> MFLIHFVHYKTILQKYTFKFKHIFLSIDKYNSLFFNISGILIWLNIIHINIILIKYSFFILINNFEYLIILIST;> MFRLTAASQKNLNSWYTKGTMRGGVPRIYYAWMRPGSFTRRRFEKMRNPFVDLETGTSLYFRDTRDSAEAIAHAADSKGIKGMDNAIDLYNEYRIVPDLYPEGFQWKHKLNTEYNQWRSNTWLTPDLIPKEHRGRFLCNFQLNIVAYDMRVVKFSPKDHRQWIYCVLYVGSGKGIAGWGRAVAPSTQEAKKEAIREAFSNIIAVDLEQEGPMYPVRVNADGVRVLLYPARRIVANFRVADILCAFGFQH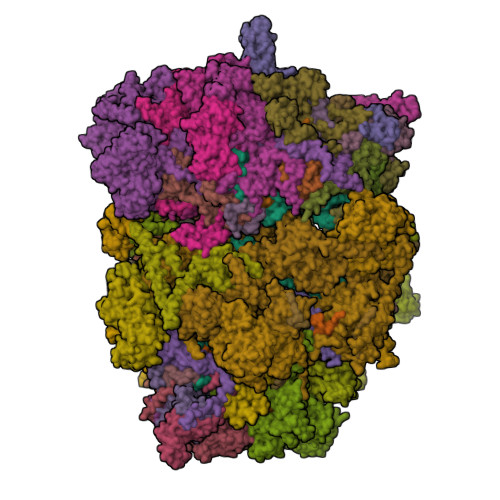AGCRINLKATNNPKSPTHTVEGVFEAVKALRSVSEIAASRGKVPHSLIYNIYPYLEEIRRRKGMMAMHPPGKDGLLMPDRVVDNRLPDHLKRGYYDDVYWKDFFAGSDEHLNEPRMGLRGDEMRRRLEEAQTSPAPTTAKDTRRRTLEDVLKRLGKTTRDLGSIPIVNPRVDVGLPTHIKRNYQLH;> MVFYSFVLVMKPRQRRFTSQALREIGVAVYSNGGLIRSITNEGIMRPYSRFRDADNTPLTYARYIILQLDMGEEEMGKVDKIIREHQDVLMALKLNNLERPVGIRSGNKELQAAYFPLDTFTRLEEEINWSPQTSADIYTQLEMNWKEFSRTRWSSFLRN;> MLRQSLLSLAKVYGAVPPLGAAQGHRLLHGKREREGSLFAVANDVKRDERLLRQQLNALLEEERMPMQARLQRNEAVSSHEAVPQTPLVDLPGVERRRDLPADPITRLFFQHKGDHALYYGTYDKPSVQDDDRVQIEKRVPRRREENLYTPIYDFCHRIREATEQRKRFVVVPSTIETRGCARVMHDHGLVAGFRDFHNDRAFAVELKYFQGDSTINVIEPCSYDGRTEFEWSPKMMRRLLNTHGIHNRLVVYICRTADNRIIDHIHAVKENIGGRGLMMVH;> MQKLLSPRTARHARLFRLAGKLADSGSPGVPKSDGERLVWVNSHVRRDKDISLSQEEERIRELMMPLEVGENSFAANGQATHGNLFYFREYPMYPGEYVPAEHNTLSSLRDELRLDLTAQSLKEAWMRVSGGVYFQSVDEYYASVDGLDAEQIGEVLAALFPELNCYEAQALVQRTLECISRPVSAASRQLSRTITAEAVGLDNAPGHYTNFLEWMGRLTETRAFKTEHALFEFSRRKFNRDDVRVMFENYRLMSKATLLADSADSYSHFYTVLKDFARKVAGEDSRHQIGVRIDEAEVDPETGIAVGRGCADGEKYHFTALLRENRDHNGIITVMGKPLSLVLDNKAWLMEMVLMPFDEANLDYRDFDAHIVSEGHAMPSIANEIAAFALRMAVANALVKLIPLTRIPLKKSGLLSVDRRRERGQFPGYLDGKKVKRRFAKR;> MVRRSHVVAYYWSRYRMPTQMPKFDGPAPVAAPQSMNSTKTNEFIDPIDDKFPMSIRGPLVRPDVPEDQYVDSWYICTSMTHHMGDYRPWSASAPPNAFRFRPFNEFDAKGREYVQYMREFARFDPRKSRGNGQKGFPFRDAYLTKMNEANQKTPPPTLETIMDRAVREHHQHARILSPLEVQRDVGRLEPIPSYAGKINADRSVFPFQWKTEDWYEYEVAKVRNRRFVFENTEEDGIRGSEVTYKIVLEGFWDHHVMKLAEDVCMFLKDVGRQIVEEKLVAVRRLLQGGAVDPELLAAFNCARAGPFGGLDEYDKEEVANFLRSDLRRLEEQCLSVINRCNVPVPGATNIYDPHTSWPHVEKLEPWVRMAEFWTSSSDTSFTELEMSTAHYEFRKFFRVIICKLPFQSTEFEKRMYDIRHWLHRQTSCEFHTIYRRNVIHDSAVFPTEHDPATPTTHEHHRMFSFALDWQSAPVNRLSTDTVHEGESWDAVAQRLGCSVGELKDANAERETIEAGVVINVPVTATRRLTSFGATPLVLPLKTTSAKDGERIRTWEEAAAILDCTVEELQQCNGHAALTYQKKESEAGEFDSSVTELVAPLSCWTSTSESEFSPVERVHANDTLVAIARRLQCSEEALRAVNDGITDVSGLDFVRVPPEARRPRRLVEPQLRPQAATDALLARTIAEEETFKLKSIPHLPQNAERFPHEYHTPTSRFPPTPSETPATQDWMAYTAKYLDKQFTISAEPAPVYNVNKLWPMQQIPGKVDQTPFEEDQTWLLHSIPVQQLEMHHHEKDLQDLPFINHEQFPRSLEWNAP;> MMRKSVTFLRRGKPRPRAGMFPDKYRRVPMLLKPQQGGQQYFNHFLIRSTNDRLTQQDVDNASGQAHSFISPQLPQMDWRNMSARSSEESIREEMRQLAENDVMQHQRVFNERMWYEKEEEHRMKARSCPEETSEHAXSNDGAVPPPRVLGGDYFKTRFGYSLVKNSEMTQGPVDYSQLDMWGEMPRYTSDMVFLYLVSRRRNTYAVAYTYEGKRILNTYTAGNRGLKGGDRGFRSEGSTDNGHQVTSMYLNDLLPKLREMRASEGRPMGRGEKVELVVRVMGFYNGRQGAVRAVQDRANEFHVRYFEDITPFPLNGPKMPRGVFK;> LFFLRMWFLYGCCLRFVLFVLCYYMSPRLPSSGNRRVLYAVFYLYNFVWMLRCFFCCFIGLVMSLFIIEGGGFVDLPGVKYYTRIVS;> MFCFSRGLWMRHIGQDVPKRHTHFVLESRLMYEKSFRDCWLHSVCRAISQLDEPLSKTVVGTHQKMLQRKVTCFQYNQYGLFKTPYYRLANVDRYHAVQGVAGTREWVPYVNVSYWTMNKMVRGGNLLVHRVHYTGWGTDSHLKKGGWEHRWNKVLQRNVLQYSRI;> MFVRSFCFLRKYGSKSKTPDLKTSFTKTTNFRKAEKISITTTDGEIVKGRGKIRRRTHSALKEAIGAMEHPAIWLWYPWRMNPEPPTPHMPQRRALKNVHGAVFNDLTPVQKKRQEQMLYGVNIPETRQMKFEEQHPLLAGALRKLEGQPKGFPFWYRKYPTRRHAYEYRFSIPVEMLDGYNDDVKKALSKGMMSIQEKQFAQEAMYMERYAEHDFDTTSPAVLAVKRALKCRVLRNHLLTNPHNNIIKTVLANTERKLNHALRRLRKVDFKKYWEIIRDHDVQDILQPPNLVTYRQGSYWKYDWNAGLAISTNLADVMDPRGLNGCVETGRSRSEVARDLGLSYTRPLHENEKKQLSHQAVYYERLAKFKMEQPEAARAMERERFVRKFSGMFVKMDIRSGAPDFPSTYRRLLGTKVVRWASKRHGPN;> MQVTETVLARAVIKRRSPQLWGAPGAPIIRMRGHHVVWKFQSYDLVVEHTHKRRNSDIRLLHYLGKHCPHPQKSLWSPDTPVAQDRHLFMLTTVDIDAFKYWFGVKRCRLSMKPWALLAKAGLLPPSLTQNSKIMPKPLFDKESLMRYYLANRKDEDVMAREKYLNYENSMVKTEEERAAERPVAPYL;> MLRRSLLAFPWWNFQTEHRQRCVLMYGGARTKNTHNANHRVFIKKYKRNAFPNRTRHHWAVSMTGVLSQRPRRMPWPYDLTSLIFNQPRQGSDKIGYVVGTSMLKTAVVATNHMVYYPKFNQRVSRTKRFFAHDEDLACVEGDLVHIKQCRKISKYKHYYVFSILEPNVEGRERLKLGLKAVPPPLFGYPVSRRIVKLNLTSTEGTQEKLAAAIQEHVQDAYRFSGPTPDQPRNRLADPVTFEDANNMIAPNAPAAAALDASDSPPLLDRGEYTEVEQDTRNKKGDDYWMNLQPKEKYDFKSFKKSP;> MNRTGGSIYAHALSQFAVCRQPWNEYIGLLTKQDSTPYHTEPQEKPAYRGRKQGREGWLFGQQVQLHYHRFPDEQLITNLSRWRTGETVGDIAMQQFRNAQPFDIEDKDPQGVQRPSPEVYMKLNYKNPATISRFLTRTGHMYPADILPLNPEAVVKLRVAKAQAIRIGLYPRFGNPFWFRSQKFRPKAYQENYDPTTYSTKRTVEHFAYNWVQTDRIRRYFRELEAVHTSGSASARGSGGGTTAEHKQQDQFYSPENQPISLHRNNISYMEDVGRSVKNPTVPGLMSTKGMKKKFHNLYSSTSTKRMGFSNPTLGIKKV;> MAFRNTFTTPGKFSTVSKNIVLLLIWRVKVFLRAEGFAHSLVMLPVSLYSKILLCDVKKKIVYFHCCTRKKSMLRRCPCVWPDGPTKSSVSIGTAFTLQKRFLKIAKSAFGFYLARRGQRKYPFLRRPHIKNTHSMNPSAPYFWSFMTAKSQMAFLPEENYITGDWTGKFFVSKRQVYTLQHATSGAKVRVKSFPSIFEFNSPSRWNIGKEMNTLTKPRMDLIDEQMLTKKQRLDYVRAGLLPK;> MLHTTRLWLGGYMMYHRKAMGTMKYSKWKGAHGGISHFYGRTPMVEEVRPNEPITLVDRRIMHYVHHSRLRHFQLFRSYQEKSNSTECKLREGEMLRRRWHRRLQKSFIAFMQFKTMKVLEDQARLVNTYGQAAVNAALGDPWNATDNVARERKSAAVRRQVRALPMVNVVPKHVATMKQIHNDRFNYRWRVN;> MLRRAYIQRRYPFNKRGPREHKSWKHHVLTEPPKPLQWRDPKVWTRDLSVMKSFDAPQWDLWQSRPRSEDMDEALQPFMDMPKSLKDRRYDIPWWANPFGAWYLQNILSLELLKLKSKTNAEKIATYRSYMRSLASGKDNTMSDDDVIRNIIKERWKTLEFGDRNAGYPCTFGDYIQFLNEWFKSLDEEGMQRLREHFDRRIRPLLAVMSPVDILWLEALTQNSPHNKEQLQRKIAFQTSLGTPEFFDMSKRLRYEINEDYKVRDELGPELFALWSKAPERWPPERLSKMYGLDFTLVRKILVWHHFKACYDACVEPDWSLPKRLFALEWIRDVRARKHGLFYGKMRFAEQKITFYSDRFLFRDLVNRREASYANVWEMDDPYRFLQTEQDYEDYWGDNYDVYRRMFPEMIGRTGEPVQQYGQMPIWAGPHRQHANKSEHNWMFAEIGVNVGHEALKKLELDPTNEKRRRFVIRQPDGTLRSAKMSEMRAWYWKEEWADFRFWAPQMEWGIENTPSQEQYQEHVPDTTDADFRKQRRIQSRPVKWFYESHYTRTGSFAGFQPLRFMQRRTEREVRWPDVINAAVQIQKRKPAAYIFKAIPEL;> MRQCVVRRYKMPKNMGVAPRFDTWNEKYEPWEHMKRMGRLVGTGFYIPPEWYNHFRMFPPINHNFQQEKTLNPHNASEPTQDDTSTLSPERVALRDELARKSRLVASEGMRYYNIFWVRKPLDTMEKEYYELKRRGVDHGEAIRKVLQGFYSGLAVKKRVAAIQAEEAKLTGRFITMREATVVLGVLAKLHKEQLTPHQVSLLAKEQGETTQSGAKLTAIVSRTQPHVNKEASSPATSEAVGSSTEESLSADALASMLSEDGEQSAVGTRYQVEVKETANDSVRQLREKAEDQTGFPDWYTGESPTYSGTSXCSRDGFALMKANK;> MMRSSSFCRRQIRPYYNLPSKSEHGRKMTGFLTPYRHWMWKQNELWRNVHEAQFEHLRRVYKRQWLESFRVNADEYIYKYNITKAAQLAQWECEMKEQEKKRIEARQMMDGRQALKKKHLDLLREFHERQFFFWYERASERLQNMNLINYVPHAQLREHIDKELDKYVAGKNEPYPLNFVGQMPFLEDGDGNIVEVPESLLSNHMAEHPDSTAKPHEPHTSSSISEAAAFEERMLRAMVSAKEEDLKEWLGDDSRALSETIDDISREEEEREADIRVARSMEETDAEREVSRRAYIERXKTGSRSIFRPPTVSEGAGGTPSAPAGDANTPMRRRKKGKLDRVHALQAHQDELLAKLSSQGLKEXVDASSVPERGKIVQSRGRIRDKAVIPTHEVLMQKPELAAGSTPGARIQTKDMVDKMYHRGKYKKSGSGDKSDGEDL;> MRSKTLKKSLAAMYMRPPVTCYTDACEAPVAMWDGAIPLKETRKLKNGVPVRTVSRTYSHPPQLTPTQLSFNDINSMYCVGNDELIQFFPEGLGGRVFQTMPPGHPRGFLYRKETHLLNLFVDKVQHWHTKRSVLSSLTNGRTGFIVDGPTGCGKSALMCQVVHFARSRNIVTLYVPDAKVWTHGEWCWPSTILPGFFDAPDAARSFLKYFAVANRATLTSWKLRCTPKDLPTEQGERQPQNLYELCEWGHRAVAPASIDRQSVCVKFLMDELSEEKKLPVVIVVDGWNLFSHETHFRYPHPDFLRGLASFNESSTDIDLYPQELPRIPASRLSFVRGLNKMILSGDDPNKFFITCTTRDFKPFDGISGFPNVETDRFANSLDEYAPYDPEKDSHFHPIQIGNFDEYEYRSFLRFLINSGELAGLGWGPLWHASSDFERKLYKIGFLSGRNPQGVVDHYHQELVWRYDYQRTRQKQYLLKRRMEGMSRGASSGAVGVR;> MVLRRWFPLLGVHRVGYTHPSTLPVPCAQRWDLRLARARIFQEYIEEKAPGAWQLEDERSMSPEFKTFTGYPMRDMRPGYGQNLPDYIMKKRLPNNTHYELFARRDIPNEDNAMYGKYLYDMTVHGTSLPSTYRMHKDINKAQRNDRKLSGNRFKVLCSSGAKNPPSGWEPIPDATEEEED;> MLRCARVALRADPLNGGSSMTLGSKGSKLSPEPHRRRMPWTAAKEYVPGVVLNARDKMVLDGVQLLDIESIDRASQLDPLEVLRAVVATREYNISTGKNIFQLASQATYNGRGQRFYRKEWQEGTYDKYVTLSAIDFDRDGNKGTAYGYITFHGETTTRPVQVDFADVPGWYMDFVEERAVPFTGIVPPPPSIGTDVPVDPHSYRLKAYPYYDAPNPPEFVERLLKDRGVLPDTPTETADVDKDPTTSDGSVHYDGK;> MRRWHRSLNPALFGERGSGHYFSTTRARLQLQAQDRIICGTHGAGIVAHQTAVNSSDNPMLSSVTTAAPAADLSRTKPHEGTGTSERDPYIRTLHNQRSAAPESSVSQSHTVNAPTVDECEMLAERWGTMNYWHNDTFPRLVVFLKKLLVPDVSPLSPTAESLLSMFEKVVIPKLTSDEEDRRKLVSLWSETTLQAEAAVTKFLFQRGSFESMLHRIITDALEKMSTLALGGQEGNLALEALKRQTLFKRNDYIQKRLIDVVSNSAYLGYGDSVWQVFFAAVEANEENLLSDRATTDAIRAAWEGVMREDVVRLPDVTGVVALYLTLVCIRESGRLVPEELKELSSGLEDGVRPGVRKLQQYPLIFLHPTVKRRFVVKAVAEILHNSSSNAFSNMLRENGLHDTAREVALCEAMNRNKELAEGDVGDAVGRFVSKGEVKTLLSSLVSGTDAVVRDAVAGIFGIGTTITIDWDAVMQNVDWSNNWQRLATALLSNSAVLSAIVKLVKNAIGAKGMSKHLFTDEYADQLQLILDAREERAASRKQRIENIAQELSSFERVDLSCDLLRKLGVDMTELDTAAAATRNMNVVQRPCIEDGLLSLVLEAVTKRHPNWVKAGVIQTTLKDPFDALRWMMHIFIRLSYVPHAGAATIARLSRRRIGPIGLEPHQFNVPAELGFVEQYDNLQYKRYDWQGWYQRMLDVHNRNVSLRCRICDLQRLDGNGVQFVDMQTERRLRILAQHRVGMGVLKLDADKYEDQADNVTFGTTKLSELLADARKAQLGEEYWPSVELKVRKPSGQSKAHYSLIDNERIEKRSGELYEKYRDAKKRSLFVTPMETWLEVKGMQVRKSVDNADEDGYTLDALQDMMDGDDGDKV;> MKSSDIFFAYRLTPVVFKSRQHDSGVNQYGLKPTNAYDYINPTNLINFGRGTTFDNLGVRRAGRGEIDSSPSHSGSPVFTQAKLIGLSGEEQLTMCQSETMALRLCMAKAGKETCERESRALDSCLGRVGHLRRAMSEACWEFNDWFIQNVSDNHTKPFQHRPHDWRHFYAQEKLVRERQQNGHAYGRRPKQFSFGARYVKTDGYGKRPRLPYNK;> MRAGCVACSRIPKLGIAALGSTTTSMQATCQETQELRCATTQMAPAVIFPLPPPLRGSYIDRKPTAASFNEHHATASFRHHMIASADVSHRPRHFYFASGTRNDTGTRSVKEGERKQLKQQTNVEVDSVAYGDQLDELSARWAAKFYGQVTFGPRNYPYPSSRWLARRFQMKKHRIIKRFRFRRYKLAAVANLPFAKMIRVGMLPELKSSKTKRGDVVDPTLSGQLVSAVKNTGEKRKGQRTRPKSKYQV;> MLKRTLTVLDQTYGPHKSYKYTYMPDPRKLAPIETTQRSEIVPQSIRPPTSYVPNHETFLERADIHRLRPTSDFKASFKDWNDLFTCDKRQLRVRGIPRMTRDAIRTAVQAFQNGNPPERFDTKEEWLYYKQFKTVDYSYRVIPELPEKYRPHQSGIDQAPLPDYREINKMPQWAECEERRQSKKTV;> MIRRRVCDGARLAPNIRATFSAVRYQSGLHTFIRDSKPSNFSSVRRSENANGDATASPGATAGENPASSGDWASHMQRELFGEVDPLGGQAHKDYYRDVTRGYSPQYAPRNFANGGAVAYPHIQSPYEYEEAAHRRVWLDHDVDRMREEFTQHRASLRSLASAQEREELLRSRAAEYQVANTVHESESVHPIQQLYNSGGTSRSALKQQAVADRYSIAEQHSPLPLTTGVDRDALDEAQRTKDRILNDSFTAENLLITHGLREKEKHDFTILQRTVRIPFQGYDMDRFLAQQKGTPYGAQQLPPNVVPSSMEEAQRTLRGSSATATPLVDAVAQKVYARNTVVDRPAIGEQLTEQIINIMRASRTTAEQQREEERAQRFGLGRQGALVQDGGPDQRTLKKHTNDERIVDAMLFQQNAYRKTPTDEHWNPYIRRSTENGVGHLLQNKFDIMRREDRLSKGEQDLTERNTIHYGVPIQQIVDEFVFRHRNARGERPLDYFKPFPNFRALRLNRMYRDVEGFSLMKQRPEFLEWELFTRYRQHHQQRRRLALLHGLEPVANETAQERDTRRHRLDEICERTPFDEREMRVNDDEMRVSVETLRSWFGVYMLPSPTVVNAVLGGSASVNLHLYHLADEMGTADTREHVLSSRYLNRLLLLESYQNRVGRGFMNHVVGRAPEPVVPHEQPQEVLRHFSAEERAMYEQHVKEQTSRQLGEWERAMKRRRWLTDHQQYGHVVSHGLETSVVDLSHTETGAVLTVSTKAYEQEIEAVRMKTNATIKVDGMVYNLLPNSERRVVPLTVQLDSGEKIDMTSEDFDRCELEAFPRNLNHALNYGIANYAYNRGNYVETQDSIWEEQTASGQEGWSPATHADGLREGLPVRARRPIFSSSAEQRIAGGPQRAVIIQYHHQPFFNPEPRLVKVAFQCDGTIMEVPISDVMIWQRRYHGPERTVGDESRRYNPAAMRRYVDVTDPFNEKTSNTEHFLDKYEPKRNADTVADKYRTTKQITEIDKWTRYDSARADNYRPLSISHRRDYIRMGYIPRYTPWEWIAIQEADQPLIAEQIRQDNIGTSYFFSLNRYWRYKASPHGYIRHFENEVRDLLQYVDGVTPWKQAQKIRTYWEVRSHHPMPQFNRPEVAMHRNTVGLLPAHMWETDKKTGKVKSVKDSVRDYQTKTPYPKWVQL;> MFRVRRLAGFIQCSPCGKMGPLKQQTRRYTPIWKSDPAVDNVAPLRDEDERRALWAEVGPISDVGSAVTAWIRFGNDPVLHTAVPTMLGGKFRNQQREKESLLPNSSSPFAYVEDYMGTNLVFGSPVHAKESAAVWATYFERRYASRLRLSRRTVANYVGLINSPEVFDDESDRPETRWSQDTFFRECAYLSEKFLKEKVSNMQQFEAALKRASPEAYLAFFDAFQQQTQTQIPLPSPSVWHYEGERRKQWAEKFISISHKAQAFFKDVLSEDVKKYQEVPGKLLQKVKPVLADVGKILVKRHERWLKGRVWTSLTEEEREAYCMKEVKRQQMQVEDGEFDPMMEDDVDDTELEEWQREHDAIMKLMNSPIDGLHFTTLELWLHTMRCEELETEHIYTSARVRAIQVAARKKLYDTTSYEEVIQAVVESIARGTLDLGAGVLRPHFNEVWCQLNYAKFGSSTITQHTTTSRRQLLFFHAGSLKDIAATATLYYATKPLSNSLDYASPYKYRRSLITLCSNYGVETAYTTQRPLLRSAANLARAEDLIHAVVTAAAQPFGERRRAATRDLHMEFQRLAVPVERVIVANPVSALLESGADPDEKPVEGEKVNMWPLGAKRVVLYKWSAPNVEKLKAMESDAASAVSGSSLTAKRLREIQELKRRGFLEVSLWRRVTAQERKQRNEIVEAKKKQVEEVVRTVPSLAHLHQYATSLYSRIEERVAFPTETSTVTETTNMKEETNKPLEDSEWEFAVLLDDRVLLNKEESVELYLPYRDANGELLAQGEYRALVRAFDLEANPNLHPAYCSVGYSESFQVFDALPQLIAQFFRVKDATAEAAGVTHIPAADFTPFCAFLRDAGLDVPLRCEFEAGQAVTTDGDVYMDYFLQLLRGEAFHQSHAQAGLTEAQRAIEPLCRAHWVVHHPGADESEWATARRSVLDHAMQHEREWWFPNEMLDVKDVVTGSTNGLTPQMYPAAVRYGVELCTVLTAEGKFVDERGSGLSARCVVNGTGAAESVVFDTANCNGTNTTSVEDALRVAHGALRSAQDRHNTLAAFRLGPLSKQSQVLLFCGVNAYEFGGKYARTYAYAFEKAKKELEATAASGFMAPSLSHEDTERLSDQPTTSPSVDRFASTTHPEQRKAQFVPRVGPGSTPLEDPAADQKSEWS;> XXXXXXXXXXXXXXXXXFVFRDPSLXXXXXXXXXXXXXXXXXXXXXXXXXXXXXXXHANTQYQHAWPLLSHDDLGNSDQSNNTKNIMYSMYMPKRNKGTAPWFRGADTYSVKYCEQGRYEYQRYLMINRFPSEYKKHFLSFLSNIRMSSGSATIPQEALHWLLRMIVDNFNPQHVHYIAAMKTLQSAGELDMARDVWKIMERQQTWPCTATICAYLDVCVEAGEKTWAMEAWNRYCTELKFLEPGEVDPKPISRVPFSLTREELLYLPKWKKHFDHDPNLDVMDLNRFNRTREVYLRMAQVMLAGGERNAFQHFFTKLEEAMLNKPTPVPEPPNPHLVRRPRWAPYEHCKSVHHSPWRLQNNGRALALGPPVTIEDEMQSRFFSNDQFLVHSVKEVLRIVLQEHKRAHPTECTRCKTEAFFYKTKDADETLKFCDDLIERLFASLGVRLSNLNTSSLLSTILEVFRVVGKESGAALLQRANEFLERKASLGDAEGSRENLTASNYLQVLSGFADESAFVYNTKKDGTCQYKTGFDPRTTMRHLADVVQEIAGNPHVTWAADMHLQVVETMVGCGTMKANDYFVRNVLRQFSWDSRFLEALYVEYRRQDDVDMWAELTKRALVWTARYNAPASERLRRLIEDDYDTIRVQTRTFRELAVFQFRDVEERRHSRDVVNELPNPWYDYVAHALPFPDRDAGYPDEYGDLGQWRAPGGPGSPVRGPGYYAPPMEGEHQRGYTAEWRDLRNPMRPPEFPTPWERKYRQYARGQHPSYDMVYAGPMPEIFPMRRDFRKPTRWDFHDIEKQGKYRTSGPY;> MRRCSFASTCRYRSADDVPLGLGSAYVWTCRNITSRGQFNPIHNFSYAMERGVRARDVKAFEKLITNPGPLRVAYTPDYLDWLHRCYKAKGTYMDARAVAEKKFNGNIVSSELSAAVNRREGKRGDTRGDTVDNDHHNLPGAPPPGMFLRPAHSFRRLAGELKRRRAQSILDEVARAQGMLDLFERQPHFPAIHIDRCSRFHLVELFKEMVLERSLDSNMIWEKALLYRAILSERKPSYPTSFHYIFTAVEDTVFAPTISTPMEMAGSGGEGHDRSSHPLAAKCPTLEAYYYYVYLVKKYYIDNAVEAHVVLRCHREPNAADLLFSNPPPKDDTEIMKAVELLRNADIQRGVAAAAAVSDPTLPPGGEGSVIGNSDNXKNSEKXSEGSRGRPARPPVLPGAYPPIDMLWRCEENLPLLKVLLFGEFNLIVSENPFVKFPSAHGFLTRPYSTDSSRTLADGMSLANVMAEKRGHLLPSLPRNTATSIDARAQDIRRLQQKHHRDDIVSFQKLLRSTHAEDSPSAFSSYSDWSYFNPRAVRAEERDRLTRKAVEALKLYDSATNDIYRHSFEDVQACHTQRVTERDRTMPPYLPTLPHFVAIIKKDPHISFLLHIGLPDRNSSEEGSAKHKELEKRIYYLARALYHTALEYHNETVRRVNRQKVNVAASLLDNFVEQEWTTILRDKHDVTDVTKTLNDTQNDKKQLARRLGRYMLFANRSLDDTGFPTDARADDYTRWMAPPSVGKVSL;> MSVSGVFSKGRGIGHEATTSILRYIPRARVPWQPSRFGRENLTAADMARLWSRGRYRDGPGNYNSGYCTERTHVLEENTVSIIPRRELEKYMPDITIGPKALVTPVSLMNARNGHRVTHDLLHSYDPHIGRLGKPAVVDHDNITVEDPNRVGLNAATLDCRGRIYRWLRRGPFFQVDNYFRRSVKLNRDGTLPTDFVHEAPLMRKIIRLAHRGHLKAACEEYRRVTTVPPVEVYRALTACCVPGAKLADAVSIFEDGDSKLFYVSRDGEVLHNLMRCAIAARHRARIMWVYNVMRGRFYENVVVRAEVDLIWRYRIAMIALEYLLDHECAEEAAAIYSYLVEEELLRCDVHVRVGLHMREAIAAGKPITLNNDVMNATSLVRDATAVAPEVARELQRRHAQTLQNNAVEAVGAENVREGSAPWSILGPLTAIGPTAEDTMVWLQQHYGDVDVMSIMRWARFRKGKDLMAKDRPQYLARAAAWIELLSKRNREMEEVPLTYMRKSKPLVLDTNSNVRVAWQTPLMRSGGPPRLLAREEGYVFHHSNSSRFVEETYRHPGESLQSRYLALQPLHTEVSAKEDFQRLYYQAQKHHKQQERLLPVSTAAIPSRIVHHSVMSALHGVSGKGEPANRSLFTXNKSNDSHSNTGVASGTSACTDGAGSATPEF;> MFRRAIPLLSANIPRSVWDPAQHNPNWSDSYGHDITNRRAWPARKWTVGLEPCTPREWLQFSHRNLAYAYNGALRACHSLPSMLLLYKEMKQRGVKVDVDTMNVLLTRAARHEHIQVDDVFLLFDELVALGARPDLAAAETLHTVLSHSASMPEEWREARRLQLVELYNNLAMEEVERLAPHRADRLLKEQMKRFRGNLQQLGSGLRPTVYCRYLHTTHTAAVLLEEVHNFLWELVPNDHPAMEIPALQLRVPFVASVLRRPSVNPGVSLASVSRAEFGDTDVCAVFLAAAERMVDADFDDQRPVSERRLFLSLLTMISYSGVLYTSDLMAQLMEMVKYSNNDETRDSDAQRVLRYALRGSSAAQDSASRTLWHSVEKVADCRVVGRYIGARNPWNPIRVCFDEQGVFKAYPISTTTTTREVSPPEGNGAVTQEQRASCVEGRTLEALNMRWDDVRRLIECTGVLVTPPSERCPQQQKMEVFTGMAVYLRTVATGRRYEGGEDVLSDGAVATSSCEQRRRGTLFAEGYDFDVWVRLFSLVQEVRHDMEKFMADHTLQCVEPEFECWEALLVTLRCALDFCVVQMQGGGARGTEREVVERLFRDVVALREELIEESRTRFGGRMRVLWLQEA;> MLSQNVAKTTVPSYYMIRTNLPHRKPQNQWEGVYYYSGITKRQRHLILLHRKREREAHMRSFNISRASVLQRLEQLSGDRKQESLPPHVRLDLAVRLAQHGLYQQATPIVDELHHQKALHAGHYALLINALACPRLGQRILHCDAQCDPALTYKLLGDENGEERAQEAYRWFDLALTSLAVDCGGRTQPSHFVPYLPQGTAAASHITNALMRTLLTCGYTHVAAIPDSVYDRMGSMGISPTISTYELVMLALSLQGNMVEAESILSFLRSHHSEHITVESFNALLLGHREARQFDCCDAIWQELVDRRWPRASPLTAELYLRSIMDHANTPTSEPLQSFANINVVEKKKVPLVLAQMDELGVPRTHLSRVLMDEVEDSLRKFQTYRSRFYEWGRAVKQFDFIEFRRRNGWLYDLHLMKCTTKQVGPLRDFNDPDAVQGAVATAEIPAFFNERPAWERPPLEETLYVTTNKERYDDVRGGDIYYDDTRGLHDRSPTWMNEVPETRYDRLYGVNHPDIAKIGIRRHLNVEYVNRKEVVERDAALMKKTLSSGRRLRHRVESSRTHRNAGSLSGISSTAGGGSR;> MRKFCHFMANCWNSARSHATYGAVPLTHSQVTSVYATDGGKVDELGLLELVEERIFSWKLNKWEMRIPPNLPNDQKELIRQEQENLKQILSEWRKCFGALNADILQISSLTGVPKDVVREKNRTWLQEEVAKLRWMGEVNKAALLRDAFMRLEAFGSRDFMFMERLCCIYGLARQGTFDEAFTNYITEDPVTNDIFVDERNPFKELVAHIVRNYSQIDIIYDFLGFNYSEGYRSSLRRYMEYLQCKTAENVRASGRLVTGDKGEHNILFDYCVSRESLVSGDSCQGIIDFLYINGNDVTLIIIASDNPWLRNRQLPHRRQMEGIARRVCFVLGIPPSEVRIRNLLLPPTYLDKGSIVRLNDIVFRLSNEQSNLLIPWLTNYNKELDPKDVDYTALAKTTNEEEWLTL;> MFRSTRPRSVGYTPVNPDTSPMVAYSQYHWHYNLPQGMERPHSVNRTFAAPFQSNHSLVNKYRGVWIEFDMHPAFSVALEPQLRKLPRGRTLPKTPAEEVIADYTALAPLVDDEKTRDLWLAKVFQHCAFQRCGGAMELWERYCHQRFTAEGATAKPPLSLVKSVLFYCNKTDNSGWRALFDRCLKDGWNYTPLFDTAQWSFMLKSIGRMGDEDGVRAVLEEMLDVQADLDRVEARSVVIALNAVTNADVYEFVKKYLFNFGERKVKFLRTTYSDLRGHGAGKLRIPLKENDNMYYHVCWHSSIRSPRQFSPRQLYFDYTPSTLGSSSHNPNAKIDDIVKDKIEKWKAEGLLPEDYVHEDRVYDRSAAFKNVARQEKWKKMPKILKSKRMGYTGDP;> MSFRYTNNLIGALKHRLLLESSYREIASRKFIGNCRGVEVVCSGYGTVLAVQLTDKAVWESFYRKGGRPTVSGGGDVSGDAETGTQGSATTTGATGDLDLDKLAESIKTALWDATRKIRSAKEAALHRSLSHNTRMRASADLKHWYEEDANTLRPLAFEALKHEAATPWMQLVQHGKKEEAAALLKEFEQKGDAAEATPTRVKDDRVKGTRTELSNREQPPLASTLKAEDSNPATIPIGSVHPLFTPALVQIEEAGGGSVSNEAVCRAQLWELSRDEQLFWERVELIRKGQVASIGSSHKRGYADEAAFAKDDTEEKVQLRFTQ;> MRCSCAFLDKSVFAAKRRVIVPIHPTPNFPAHFIKSAFTTDPLKEKQKARFSSGGEAMREVQDIPKNLEGERSRRDLASRGDTEFQALVEFIEGASYDQLISGRRFKKVYDVLSENDDMFIWLCHTAMSVLNPGDMRSRLIYNHLRILAESVASGEMTQRTAFRFFESAVRSPAYREIAKRQLEGGAATRLAGISAAADVMRRMGLTRRPMSSYFELYQRIVERSEAMTPWGFPPLFQFEERLSLEPRLKFFSRASQQSLERRRRGHVMTPHTTLHGRRIFWIPPTWNRAGRFLGPHVTLYPGMTPD;> MRRFCTARVSSYVKRAPLLLPRGGRRWRSGAGTTADGGGEKEYIADSFESTAGSNAYAAMELAAEARREIHELWLSAETALEREKRVQQVAALIEKYKLDPSTPREADVSRGLGDAFDRLLLLCLPLGKTDAKGTDNLERLMHLAGRNGRELSVRTIQHLFARTDSFAEALAVFYTMRRCHVAMNMEAYYSMLYSLQRLEEEGWGQHFRNEYEENGAPSEQAMDFIVKGISNALLPENKPWLGRVMFQDRNVPDRRYDTRDFDELDTAWTQRYKSGTPAGAH;> MLHGTPVRRASLRYRRPYWMMFLKGVDNWKIYTVIQQPDHQRTEMLYQAWLGGLDRPYTRPKCMANQPLWLSKKRHMLRKERLDGPETPLEKYVLEWHKKFHSFQGTERPTPDDLHTALDLVERPLDLSYALQLLGQCRNLNNIRFAKETFLVFLEACLRVGRRDCAEYALEHAEPLGFWFIDEDHRRYLQGEQTWYKLSPLDNLYYPVEENAKLNEGRKPITRLSPATESPGSGTAISDGEPSTDVEGETTVDDEIAQLEAELAALEREGGGK;> MFSESLCILSRRFRYNTKFPALVSYNKLPWEVVNHETPQFHMHVAPHYEQLLTLAASSPVPHIIGSKHIDVPREHRLRLLPGMLYLLDGDTLPGEFTINRVLDPTALQYYGRLSSQIVTVEAVRMLVPDDLRLLCNCITFKGPLHLPVAPYASLASLRGASQGGTTGSETGSNCFTLYHFVRPNRPPKELQLEKYYIHAPCVAPLSEFASNSDERGNWRPRLQAPKRTRRATPLPAYRPPQSYLMGLAERLAVVPGGCFGRRSLMWGHWF;> MLVSYLRLQADRRTRHHMMVDGQINPREWFNWHPKEYQPWYFDRHKFLYEQRQYAQFHHLLCHQVYLKDMLHLMRYPEPYTHIIDCRTSTQKMHRWVPHSLWLPRDEVEYALQLSADEFLDMYGFRKPDKSDDVILLSHNGIYSEQAGWEWKKQFFQHVYNYRGGTNELFGESYSDMNVSDVLSPWKGPFPQSGVFVDKWSKRKVLTRTGPFDRQYEMQDFALPDLELEKARHPEEGPRQNMPFGLQ;> MRRGALSLLKAGLLGHYQQEAFEARKRFEESTTYPGPIRAATPGDTRFYSGSLESILHDTDRHYWRAVTDDPRVQHLIPLRIRFKIFTWVTSGWEQRMQVVQIMAPKDSTIAQVKDLVIVENQSPYLCVSSFHLAIDGKELDPQKTLGEYGITEQSQIDAIEQNDHLLHRDDERPRDWTVDEITAEDVKRSPYKEMEMQPLQNLAPRYEARPKGYFGRTYYSGMKQSS;> MRRVRDGLFLSHPSSALQCSVAVVSTGEFDHPPFQFRQRHTFNTTPLHDANRFGGRTAYLREIGPVNIKKQGRRFKKDPRTVQFNVDVWCAQQTLRKRWKQRDWEVIEIPFRLVPREQQRVIPELYTDIPQMTDPARNDFSNIRNKVYDREELQGVLFPAAGAMLYPPLQRVDKQAMTLDKYL;> MLRFTHRALTATPERFSVLGTTHPKPKRTGFGRNNKMRSKPSDNVAWYDKGPVEWLPRPVRLTYDHLDQLQQWTMRATLDGRTEEFNRIRDLHREWSQHPLMPVLGDVEPKFPLNLFKQNHRAKKRFLVRWHKANTPANWLWMPRGPTVVTPLHRTNPTQYPENWKQMVQRKSGTGTPS;> MFHRAFVSSSDLTGCTIALSSVCTQKRYWAKPKKRPKVGQGFHEKAQKWREEYLLDRHRALADSLRAYVEFSTSKRVEPWDARFKPFDRIEKDGVYVLMRYMMEEKLQLCNYHHRPVKRLFCNIGLMGPQITTKARWKPYRFATNPAGTSKAERMYQRDKTVYTHGHND;> MLRSTLTSLNTFLTSSVATPPISVIRTGPKWWAHPERMVRQKLMYFTLGVDQLPLRRTAVIQRDLQRFHMCKPPPRVGDSTGYKRSRAAQLNTWYRRIQYQEYHMQHLFTRHVWGLLRVYPGNTTKIQGKADDGYVGYDSVPFHRYNRAPLPFPARELYERRK;> MLRRSILFRMKYADLELTTRGEFPHGMKEPAFVKKLDQNIPWYFSTYRSMYHWPITGDNWSDLNEAEKHHDLHMFYTLAWWKLGEGIFGVDEDS;> MFSLTQTWLIAHWYCGHKFRHRFMRDKRFHPSLQASHDARNRFSKRRHFKTNRWNYQQAYRDMP;> MLTPTRRLPKALSPYAQALRHVALRGATAFGPGAKEMELDMLRKGTLPADYRPPVQGRWDDTIERWAYAWQFPAEEEQDDITKSVERNASGMQALLEIGNKLLRSPPSPEPLSGKASKLYPPVGDMSSGNTALLPPNPTYDVLEQDVSELMAEDAVVVTSQPRLRAEELSAKYNVPMAYIDDSSEASNASKSLALVMEDVGLEFTEDGLTVVISALSRQGYGTIGRAIFDFASAMGLGPSAEMYRALMKYASRRGDVNESMALIEEMKGNGITPRIGNWHELMYTFYKAKDYPAVSQIVDNMKMYANIEPNEVTFVLQLKALAKDNSQLNSLPEAIQLFDQMENVYGFIASRPHYDAMMFHLSQSPRPEMRLRCEELAHKMELMGIVWNANTYLNLIRSAQVVGDVAAVEKYLSRMREEGIPASIGHLTWAVQAHVQSMIRIDYDALKEKDESPLPTWLEHLETCFGIYELVVRRGWVMQLPFVNALLRLTCQATILSMERTPDEAETIGRFEEQANKIWNHTFDEWQLQKDVYSYECYIALLAHQQRIDEAEKLFQEMILKKDLSPSRRTYHCMIFMHLSSGEEGGTARALRYLEAMERAGIQVRPSLLKKIVRVNNAAGYKRDMKRRARRIMQAREEYLARKEEGVSFGEGGKEGASNQRADVDAEGNSILEPLAVSPTSTLAWWEKWKRETVSKHELFTEEGADGTPKGETFEEKNEALRMMGITSSFQTKDLVPQPDRQKLLPLIRREEGEIAGSLWAMDGGELSYPKDGGGPQGWGVRLWRERQLVKREYQKVLDGYRPVPQLSTLGNSVRTAGDQLDIERSGAQTPGELSDYRNFPDNRFDGGQLKPESEAAPAVPFSAELVWQGEANDKLSPYKSDEEIALENDNTFFSSLSKETEGKLSIAVKAMQNKEENSVDVRGKGVTRRSKFDYLEKWRDMYRHGTLEVPEGPTLNFGRTPDDHKETMAALVRGWYQRNRKEPASEEELKRWRVDEQRSSETSASRAALKKRKQVRSRHRNK;> MLRGWHPNSSAMQVGMRHITIGGRHSRGGFRQPLGKHPQVKQGTVEGVPRRIPGTTKVTYTNKKGRTFSFSVPVSELTHPQVTLESAAGTWREMDTSFCELGDIEDDMPSPVDECLRGGSSLDKRLIQEVRERFVSFCREYVLMDTSGMKSTILSTELNAGPDYEHYDRRLRRKRHWLAIRHRFEDVRYVIWPDVVEETARGDSAQADVSLTNPSLTAGEMLEALLWLDAASTFCVRKVHPSDLGDKSEFLPLDLQREVEVVACHARRDLDFFDPSATSLEQFTACAALCVNHRVPFSLFFPAQDVCGDASVSTGQCIVANAPSPHTALGAVRIMALISEGSGSDIGKTIMFSDAFGAVTRFGILRGLSRVMSVEAFGCKDALENVNESELCIILHFCAEVREQNAAFFRRYEASEEDSDPQQVSFLAKYQQLSQIALARCKRLLYHPDSPRAQVMSEDGYIPLVELQRHAEGTNKAALIHYNLGIRSAQGMRRVALGAQSSARLAELVSRLEEASARVSGNTLVNDLVHHLSHKAAAGKMSLTLREVNTLLPLLSRMRRESPNGALDARFDRVFNAIDTAIGAAMRHNCTLDELLDLAEGLAACEMVPSALKQVEMVLIRSVMMHECSPMHLRRMLQAMFTLMRTSVPQVLLQSVASRVADYIKEASHMDSSSSNGGGDEKVKNHEECEQLLELLVVLGKCGYGALPGLVTIYWEAQLIDSMQLNPRLRCSYASLLASAAFALKKHDKRAWEGLADESHRLFMEYTRCNKENDIGRFAECVTGLAVLTQIKDNTNSSDVAFLKEYLSATSLELKSCEVIRVQELTDLLGRTLEWSEALGVVAPDVVIQLEKALFVMLENVSHTAPGVGIPDELVTAACCLVDMSSASLELRKAAAGVVGGAIVHAEEALETLRSGAPTQVRPGHSFDVAALASAERENVYKNSILQYCAALQRSGMSTHVEELWS;> MRHTIPFFRRSAFVPAPGSSLLNPRSQRAKVRRMVAAQKAQGENFERQALYAELGGSPSARAPRSKGERSKEATRRVGCEVAERAKHMTDAEWEGVPVDEKHAFAKYMHKVLQEHPTETTEQQRRRYFETTMADVFELDPRKTVRDEYERVKLGLPVHLKNPQYSLGVSQAVYDAADASLFDPENVHRLENAMTHVKQVFADYVHKKREGVSTEAERRMLANLTAELNLETQKHLANMFKYAEMRLRQVKLEERHHQLAEIERLRRMAQQRGGVKGRKGGSRKMSRMERLKRVINRAVGLDIAVAETVLTEMQAQEEFLQFCEVFARLTLGSGFKHTGKDENLSAYIESLRKLYSMDAATLSTLDVVQYYSSKEGAHPVDWAKRWYERALLLPLQSTPEYQKLLQIQQRDESTVKHIKETAGTGHAFACEAEAEVARIKTQKVVNLVEKMFMDPKDKRLESLHEKRLRYLAHMQMERQIRCVRENAKLFDGVENMPEAAQCRELYEKIMEKKTAQCNMTSPPEGEGSAIQSAKTEGDHCEVGPGMFNVYDDAEASSLFEKIREITLRVIRDRRVQSAAATKARMLNRIIRSLKGGERSIAEELRALHQQRKEKMTMRILGIIENDVKTEMEWLQNMEEAERPPLLPIPENMSYVSAADVQAWRELREDDERKAANPFERRRRTFQPELLGQAWSVPNKPLLFWGTGVSAVQQALRHVAEDAERKRQGLLLAPPYPCAENPWGWRLAKDILDDNN;> MYKKALHSFFLKVHPDFFHHNRSQQTVNESSVARLNELLSWAKAFKSGHLQPPPSSSFTLTFYRKPDDNMGNGETRREGSGSPVSSLVGRSMGDGSLSPTIIQSTFELPSNFAPSDNHRGTVERAVNKFLRDLLRRAACIDSVTESISEAEDATAARAEAKPLRRRPRGSQHRGAPTGPKSLLDEAVESMTVQWSLTPAPTLQELIEADQILFSRDLSPLQSAAALSTLQRHLGELNYSAWESMPVIVSNQFSIGDLTGTITIPWDFTPEQFHSFMAHNEKGVARCREVAIQYASTIEQLIAELCTALELDDILVSCSHQDALRLMELLHRNRELLIQYGLSKLTLEVGNRHATRANGVVIINCSLTSEQLRPWLKAISPKLPLQQRLYELSKQMLESTLWHLKEFRTMVEPGGVDAFSNDCTYAERLQWSKELFRIGPSLAPWDWSEMTFVLSPDVDIDWANGLLALPYNFDGDALVRYVEEVQQEAKSRKREELLAASAMQREEEERRRKQQHDEELMVECQEKGERSGDDSPTVAERMRHLYRQTNPHMDEYLASSNSRVDTLPVERPLSHAVTFNSDAEAEDQLKWEGFYAEPYVDQAPTSDIDDMAHTFMLTNRWHREEAAKKMLDQLRGTYGKKSRRFEYQKMGDVLEINNAKVQPKGFPTLTRGIKPGC;> MLSHAVPRLRLAAAAVKAAEWYAAENRRKQKGGDVIREKVDCTAPLWFDDTEQNLLAREQHVRSPAYRELHRPALTNAAMGLYGGEPGFEKAHRVWVDPDRPHIKHIYNQTALARNLRYARYGYFKRDMHLLDVDKLVRHARLLPTPGRLLTDFLYQRVPLPDKSCAALIRYQRQQIEMLEVWGRHASFQCAVEMFERMIVTNIPPVEVGVETHGEMVLCAAACGKWEEGWNVYANRARELEKESPESFILNTFFFDALLTLCVAAGRVSEGIDTLEEVIKRNLRPRGTMLNKAMILYSILGEQMSKHEASRATSEGERSYLCEPEEVEKMGLEVWSLFDFYQLPRTTASIEAYMRMCCAFNKPTLVLKAQGFADASDIRLSIECFHWLVYAIRGVAGFGDYVMDVLSQLRPRGLTPDFVLFTLSFMYCALQRDGELALAIFDQHFVHQNMNPTPEMVLLFIQACSNCEEPTAVMLERSETLIKRLEAVGSSVDLISPIYDQFLELCAHLGAVASGFSALKRIVGFGKPLTTRMINSLLLANSNAISSNGSLSMTEELVGFFTLLKIRPNADTEICVNLCRDAFGESPVVNDFIKVIGESLQGDSEKGEAPQYDEDIPVIQVPPHELRQLRTEWKLSPRDIVLRRFGQHTKPPGKAALDVGSMRGSVIPFGRSPGEQLV;> MTGPTRALFLSSGINLGRLRLAEQFSSMNGWQSKEDPAFDAYVKERRRKENYEAFDQRVERGYAAAAKLHKAEIQNAVKRRLKSSGAKFTAETLREMSSAVTERLAWLRDVWAQIDADYRSGDSARQETAAQEISAALRGEPNDYMRWVYETKRELRFAGPVGRRAIQEELQAAELPEVLDEEVNRYHDLKLNMMEIEREVKAKYGVAGQQHWAELQAAKDEEYIQKLDEAAEVYKQLLDQSARLDESRRSELQRSYVERVHQAQVRFKAAMELEGQREQLIEAHQAMKEERMRTEREKRRQLLREAAELRAQGKKSADVLTALKERQLDANAKRQAEYELKECEDILKRKSEMLDMIAHFKHDVEEREGREMLQRQKSDERQVNVFGFYEEVGVEDGLSISSEGTTSQGGSSGLGTVSTSTSCAKSADSNSSAQPSQKLRKEELWKVINADTYEDPFRTVHQARLDAVKTYDPAYARTFPLNLVLGRKYSRQGAGEMAAGNETDKQILQKGNNILYSFQWGLNNGTVHDLDADGGTDYFMDGAFHVRDKETGDIDWRYEKKRGGPVFRGPKFYRLGAQREAADPGERAMDPTPYTSTPREHKWRSS;>[2x]MSAIKRSLNVGVVGMGNMGVPIARNLGFKARSAMYLQIHSRALSKAKRVCDDLSVDGATCAMRIHDRYSTMTKWCDVIVLALADVKASRHALLEDNESLIMNARKGQIIVDHTTVDAETSRECAHEAARRGAYFLDAPMSGSPRACFNGQLLLMVGGDAETFQKMLPIFHMYADNVFHMGESGSGTAAKMISQALVASHNAAAAEALSMAHALGIEDQSKLVQVLDASWGSSTMLRRNAPLLQDLIRNPDKTPPTSAVSVDRLLSDLAHLDASLPKRGGEDEPFPVFDAALRSLAAASDAGMGDRDLASVVHYIEAGEAELRNRTHVPLXGEHLTGRTAATAANSSVNETPSTVNGSSEVPNEFGVEDFY;> MTDPVRRDPTEFLRVLRRMSRTTSWQKTMLFASKGRMVGYRLTREHYNTVLFSQSLWGRALEIVRVVRAMQEDKVQPNGATYYYIVNGMGNADHGWNYDFRINRRLEKIQHWRVALEALEACEANGFDSTDTMHNSALITLVIPGFNRWQQASLLLQRMLREDRRMHPTMVKFYHDCLVRNNRPREASSLMRLAAERGVHGYEDKWEADVYKGRPLDSEVMNESEGNGLRRQASSLAFASLMLRGDQRPLPENLQALLEEETTRNIEAERSVPVPFSAGLHATEINSVFRPRVYRQLWYKWQHIANRYRPTAALKRRQLAPRDSPTGIPGFYRI;> MVAKLQHNSAPTTLNFYEKSFQQLSDVQQRQTGLLIGAAVGDAAARALDGYTAEEVAAVAAESGSLQDEDEDPVVFASVTPREHKSGLLRHHSYTFYLFSQLLRVMATSRGDFPVQYVKNEWVATARAHPDCFVREHASLLHVLCITMQLPVIYPWADDSTLREYASGFLEFLTETPAEQAVASREDVYAYTNSVLGVALRCLQSNPDPYRNAAFMAAPGTAHVFPDDLALYCPPALVGSSHSRTEELSETDSETVPLFPARLLESDVRVVRECLVVARGAASFAEGIKAAIHLGGPVCQRSLIVGALLGARMGVRRIPISWLSATYDHVPLVTLALQVAQWSWNPPHH;> MSTSSRGILIAGLTNRARTQMAEGILRRLTAGTIFIKSGGVHHESTIHPLAVKVMKDIGIDISKQSVTSLEAARRQQNTYDVYISIDCSYERRTLDKSQPPRAEVRRRESFTVEYGDDGSGPRGGDDPVRYDPLLVPRTPSHWSVGVDATDVRRRWQIWSPRDPSIFHETSTRKFQDHLYEGEPLFMQLRQCPWRTQAKVSERWEMDEVAIRYPVERHSAHELRFVQAREQLLQRSFDLLTKLEKHYGERLLLDRALLEEFIS;> MHPRLSGQGVFPRYGGGWMHQFGHVYALQQELLNAEANNWFRAMELWHTARHEGVAMNVSHYTNILRQCVPPTAWEASLMVLKQMRRENIRPDVVGVGCALAACADANRSEEVEKVFSCFSGKLKLDSICYLALIKAKMSRGGYAEALAVGREQDADGVPFLPHTYTHLLEAAEVADDGEMALELARRMSSEQWPVSDRGREALKKLSTRHHWEEVAEYKQFVAVEDHKLSLPPTLPRG;> MRRKTTLNIGQVICFSSWNDGSEGYEWKSRALSEKRSLALEFLGNVNKRVSIHDAIRLKADINKKAISNVSCPSFFSGIEGADEDEDQSDMSLCSLLGVLEGEIETDCITHLSPSDASLLKEEFLCDYDPSDTKRMAKWVNLRSETSDYQSYGAIPEGERSLWSAWYLRNIKAGKKPI;> MNCSSTLACHAVVSAPSTASLITSCWTPQQHCYRQLMKSLRAAYFHDRSKLFWSRHRVLVEFYKYSEEANEEAVKQLVAIGLEVAAFIDHHMRTDVERIVKHNETMMALPVAQAKKFRSDYLLAEKQHDSWCKQKIKNIMKRRPPPPYPFF;> MQRSQLARKFATQVGAYSLLRGRCHAVSTWKVMATQAVTIPMYLPVRFHSEGHAAGEEAGRTGQYLLNKDDVLTRVLEVVKNFEKVDASKVTPQSHFVNDLGLNSLDVVEVVFAIEQEFILDIPDHDAEKIQSITDAVEYISQNPMAK;> MRHFGPSIAHFPLSANQLRFKASHIRIANRKRVEMFVAKRFHLPTRLATAAPDIAAEWHDELNPMHMYPAIIGIGHVQPVWWKCAICSHSYQMSVEKRVVRGGGCPQCVVNGKRAVADGALEGEMDSQLRPKRPVMFNMRTKY;> MKRIFRSSVRVGAALPLGAVVPAIFYCNGIRIMGRQYTHDTYRPFGDGYKEVRGTAPTDECNLLFASLNDESLPLCEDSGNVVNGQLVRASALVDSDALADSQELVDVAIEEDRREEEDNSVLLVPXHEEQNSVTKKQNEGEDVTTRCDHLFSVVGCPTTVSTATSGIPNTPSRNYLSEQDALYLSPTTPEEARVPSALCPQLSACVMVVFAANDMRVHDNYALALAATRAEAAGGLPVIAVTVVDYRMFAQPSAVGGFFRQSPMRARFFLETLAALRYKLERELRIPLLVRCGRPEDHIPRLVVECGAIDVFLTTQYAPHEKEVHNDIVEAINQRRWVSRDPTAGYKAIEHDATVVHPFGATSASTKVGVKESRLTAAPVAHSVWQTTLVHIDDLPVPVASMVEGERWYHDDVTTANIRPTAAFDRCINRLSDLPARGDLLPTTGELSGLEPPPLYRGRAPTLVELGYGSPEAFIEEEVIATQSSHPPGEDAAIERVLDWLMDGGMTSMLRYGRDRRTNTKMYSQRLSRLSPYLSCGALSPRRFYEELRRFTSEHLRDNFVQQQYREALLRLSRRDYWHWMGLRYGPLLFYEYGPRPEHTDDIADWRHDPKIVQKWCAGLTGIPFADAAMRELTLTGFVADEGRQGLIWLLSRGYGQDWRLGAEWLERCSIDYDPFVCYGNCAYYSELVRDDFGETVRNIHWLAHHHDQTGIYVKKWLPQLSKIPPVYIHRPHVLTERMQAMHGVQLGKNYPYPLKLWDGAQYTLSSEHLTTYFSEGSQWHRKAKNGAGGSGYAEALRHGTVILEPHQLQSSAFGELEHGVMHTVPVVKDDTAGRGQHNRSLTASDE;> MSKSLQRALVFSGQGAHRRGMATEYLRIPAVACLWERMKGSMEQKYGISLQDIITENPTRLYVYNDAYDVAAICERSCQDGGSVVESTPKQKLISHPQGVLSLTSLTQPCMLAAHMVSLEYLKETRGYSVESSEVIAGHSLGEFSALCALGVLSPEVAIDLVYRRGALMEDAVKHSSQSNEGHLMFACNPQRAKLCVEDPDLAVDQLHIFVELIARNLSTTASFIEVVNYNISYEQYVVVGDPIALSALGKCLDPQFRATSCGSSATLDNIVRTAVSSVLQDKQEGITMNPNTGPAPDFVTSCARKYGIRSTFRRFLRGPDDGYTPSLEELTHLTLQEDGRSGLKKKSWFIPLPLSIPFHSSMLRRAMDLFLPVVRDALPDEETMRSFFCIPQCGGSDXGPSSRCASEPKKPVWLTNLTGTAFRPFDVDFQRDALDAMQSMNVGEIRHNGRYHTNLVELAFKNGMDTSSVRDMCAAVLAAQLAHPVQWIDVMDSAVFQHGVREAHEISPVRTVADMFKRTVFRGKTSDASVGEAALDIVTRCLPSEERFL;> MWQRLRFDRLSSSVRRTNLNPLKPCAALTEQRAELRNLHQYPTARHKSLVKDRLRFARNWWLTGGNNYELVHEVGHEREATECFAEYAQDSSRDVYLMSTNRLSDLPPGDRLKAIVGLMRSRWEVKDANRGYDKAKLLLQALECFSEMKASGQIGDFNSLPEPDQDTFLQYVEGCSRFAQACSHSHPDAVRVLLRAAQICEEMRCVEKRDEMIQVTEAAANRMDRAYAFSRPHDTLRAAPPSLHENEDCVRLKNTEELRRRFGNTAPHVLEKPKRVDCLRIHRNRPLLLHPMKDNNKLLELSKLPARPEFDSWTSHQT;> MRGSLPLLFNPVLPPSTARLRLLTYPMALAQPHATVPLIQPTIDGTHDGRNGATVSLRTQARMHGTADGTMATAGDSSQNNSVMDSPRWLRNPDELCVAALRRSRDVNKINSYVATYKFDDPQWAPLLLPEVTLRPQVNSTGDKPNGGNEAAADVVSVGPSVSATPESTPPPPPSSSSSSPYSCPADCVSISHNKMIMLECMSRHVNFSLRHIVQKGHGIYLIYHAQHSILQPKGLVEQSFVTCSFGIRGERLRTDIVHVGPIDAADVMELQPSEGHDHPRCCFNLYQKSDVRRGVIAVSQVEGYGTWFQRKPMLWQRSRRIGALQSQLGAFAYDLVDPHEVGKWRDCEVSLLAPHMRFFRNGLNGAEAVGIIASSQVAQQRRLYLGEFEAPAITALDAVQQLAHASALRCKLVTPVVDPNGVGGTGSGSLGDENMDKHIDMETLLPLSWATRTPPPYVPLEADLPFKLQMSRPTVFAESHQQNQAYPTGGTVGSPFVRGAPMMMFEYNMHQGVDHYVYDDAPSARPMKWWSQKSNMPYSGYMYFARSGLVDRFTPSEDIPNPLEPTSKRKPLHAVVPPTKVVQERLRKYRRKQQEGHKQRRRASSGSGVSNEPDAVNRQESVSRGTCE;> MQSGLCHCVRRVAALGSVANLHHFTNLPSGFSVWTSRRWQSQSSRGQPGLQWQEGVVDPRYSSSGNMRRFNPDTVAHYVKATIQNDRREMGLGEVYDWHEFAKDAVYIPTRSGPLWVGSDDPRCAKFMRRRSKMQKTPQQKARPKPGPDPAKALEDHPLREYFTTATNLRDPLSTANNLHRAGLIREYDIKYTAAKVRYVPRPPVVSIMGHVDHGKTTLLDYLRKTNVASQEAGGITQNVGAFQVKTLGDTLVTFIDTPGHAAFTTMREVGATANDLIVLVVSAVDGVQPQTKEVIELAHKSGIPFVVACTKIDRQPRVENVKQQLRDCNVELEEDGGDTQFVPVCARDGRGVPELLEAIALQAELCEISTPKPSRCEVTVIETNGVNTTTEVAGIVRCGKVRAGQVLVAGMTYAVVRKVLDEHGQIIQEAGPSQPVVLHGFRVHPKPGSILLQVSSESHAQKFYHFMKEVYQAEGRREDYLQLLNQEQHGMLYARKPDNNLVRTYSTQAFVLSCKAATFGMLQALMKSIYEIPRLEGISTEIKVTEVGGLRDYDVALIGSSGQPGCILLYGGCKDTNTLDVPNHVTVIRFNVLYHGLEALKETLVGALPKITKIRVTAEAECLQVFRASQAGKSGNAGGMRVTKGTIIAAHLTFRVCRKAPLVKGTAETDGVSDNEGDGDEDMLGHRVVVYEGQIKELRRFKELVPSVELGLECGVIMQDEFQFRTGDILQQYETYEEPRDVAEEYQKAELREKIMRDTAAAEALLAESTGGEDKPTEESEVKTTI;> MRRSGRGSAVRWSSLCKCQCCLYRTPLGGTYFEQALPRSLGARQGKGVLSTVNTALSRKALKRRQSLPRKKLNVPLTAEGLKERLKQLSAEERELSIKNNTEECDEPSPNEFTTTHEARVALARVLHHGENAGERKEVAMRIPSFCRSPAVSETQSIVVDDKEGDITNAAVHVGCSVLGSDLDHLERDMIRDYHQRGKKLPTFDNIYRTLGCGRKGTSVSDTEPEDENSSGAIQSECGLGDAGRRGTVVVAPSHLHHSTPPTKGRSGEEEEEGGCFDTNTLPADANPHFPPGACDNEVLAPLSGGCAASEQTEITDTASFIPSNSRLSTAVYDAYRQRPADDRLVVLRGTDFWDNEENRARLQELTDYAEEDFAREMLMEGAMDTSEVGYSTNKVRKETLLYFQAHPINEMIQEPFARVRSILPSDGGPEVHFPADDPDTDVDIPTAQARTMARELGLDLIRVGTLYTPINDRRVVAVCTIADHREHMRDMIRFKIKKLGVQRPPTKEGIEVPFRGGTHPHAVRFKSIGIAKHLLLGHVVRINLTDFGTVREGFPVFGSILDEVARQALQLHAYHTAGVVRANYNEVYCYLYPSTGRSPKSTVLHPTQEQLATVRDRCLLEREREVYFDGLYDKKTPRERLTYMRKLQDGTAWADRDDGLSLQRQRDMKVMLGYLPKGNHELYAARGDVNVPAPFRASHPTSVDRWTHPQESNLEQAARGSAVLAKRLSMTVSEMHDRQETAENPATLDRFYYRIQGPALEAGELKEALGLKGNRKRLPRRAPGWATLGMEKVSPQEPGHAAK;> AAAAFVLFMAAAA;> AAAAAAETDWKVIAA> GPLGSKASNNDDHNYVYPLPENMVYRFNKSTNILDYLSTERDHVMMAVQYYMSKQRLDDLYRQLPTKTRSYIDIINMYCD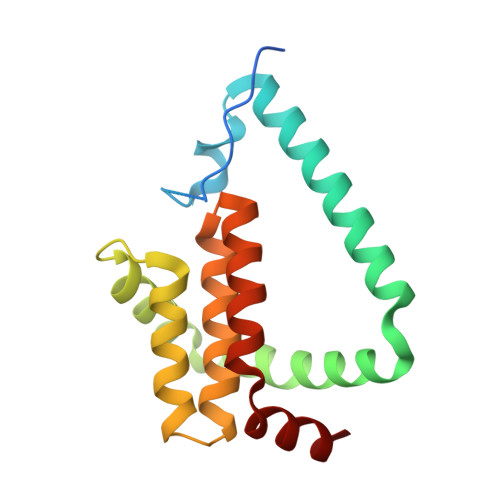KVNNDYNRDMNIMYDMASTESFTVYDINNEVNTILMDNKGLGVRLATISFITELGKRCMNPVETIKMFTLLSHTICDDCFIDYITDIS> GPYAGPLERQRPLKVKAKLPQAE;> GLIVDTRDVEERVHVMRKTKLAPTVAHGVFNPEFGPAALSNKDPRLNEGVVLDEVIFSKHKGDTKMSAEDKALFRRCAADYASR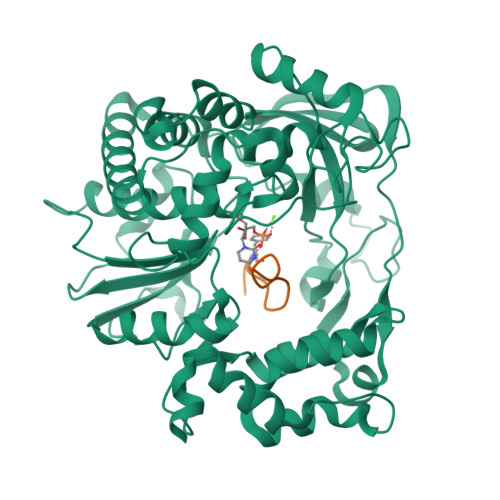LHSVLGTANAPLSIYEAIKGVDGLDAMEPDTAPGLPWALQGKRRGALIDFENGTVGPEVEAALKLMEKREYKFACQTFLKDEIRPMEKVRAGKTRIVDVLPVEHILYTRMMIGRFCAQMHSNNGPQIGSAVGCNPDVDWQRFGTHFAQYRNVWDVDYSAFDANHCSDAMNIMFEEVFRTEFGFHPNAEWILKTLVNTEHAYENKRITVEGGMPSGCSATSIINTILNNIYVLYALRRHYEGVELDTYTMISYGDDIVVASDYDLDFEALKPHFKSLGQTITPADKSDKGFVLGHSITDVTFLKRHFHMDYGTGFYKPVMASKTLEAILSFARRGTIQEKLISVAGLAVHSGPDEYRRLFEPFQGLFEIPSYRSLYLRWVNAVCGDAAALE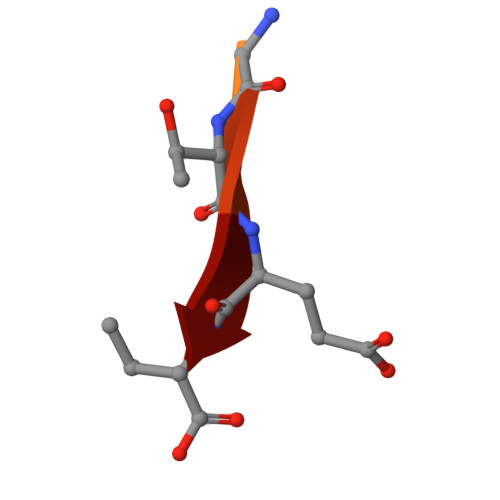> NNLQDGTEV>MFTNFEQTIVDTTEARINLVKAGHGAPLLLLHGYPQTHVMWHKIAPLLANNFTVVATDLRGYGDSSRPASVPHHINYSKRVMAQDQVEVMSKLGYEQFYVVGHDRGARVAHRLALDHPHRVKKLALLDIAPTHKMYRTTDQEFATAYYHWFFLIQPDNLPETLIGANPEYYLRKCLEKWGKDFSAFHPQALAEYIRCFSQPAVIHATCEDYRAAATIDLEHDELDMKQKISCPVLVLWGEKGIIGRKYDVLATWRERAIDVSGQSLPCGHFLPEEAP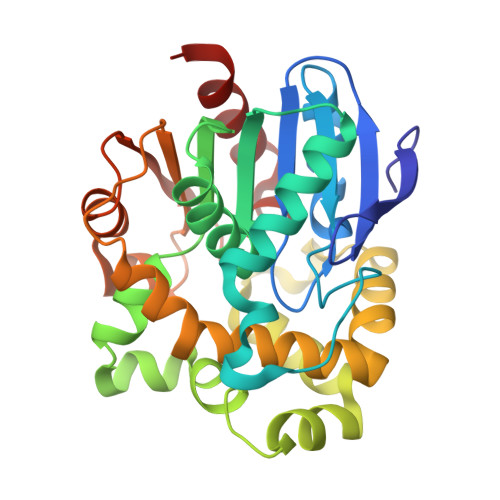EETYQAIYNFLTHC[2x]2-(4-chloranylphenoxy)ethanoic acid | C8 H7 Cl O3 | 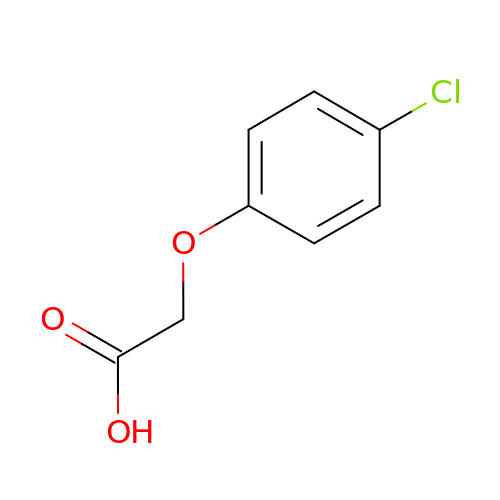SODPIMGUZLOIPE-UHFFFAOYSA-N> MAVTDSLSRAATVLATVLLLSFGSVAASHIEDQAEQFFRSGHTNNWAVLVCTSRFWFNYRHVANTLSVYRSVKRLGIPD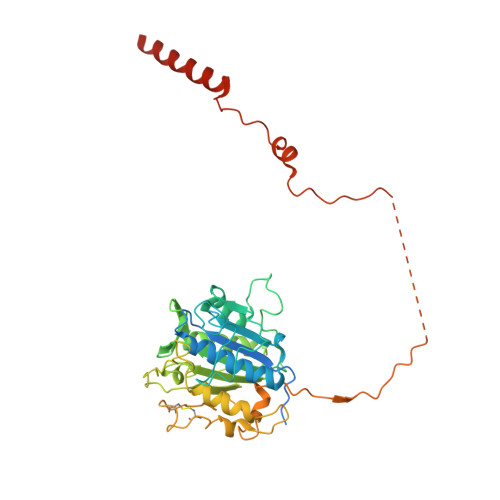SHIVLMLADDMACNPRNPKPATVFSHKNMELNVYGDDVEVDYRSYEVTVENFLRVLTGRIPPSTPRSKRLLSDDRSNILIYMTGHGGNGFLKFQDSEEITNIELADAFEQMWQKRRYNELLFIIDTCQGASMYERFYSPNIMALASSQVGEDSLSHQPDPAIGVHLMDRYTFYVLEFLEEINPASQTNMNDLFQVCPKSLCVSTPGHRTDLFQRDPKNVLITDFFGSVRKVEITTETIKLQQDSEIMESSYKEDQMDEKLMEPLKYAEQLPVAQIIHQKPKLKDWHPPGGFILGLWALIIMVFFKTYGIKHMKFIF Aichi virus 1 (AiV-1) is a human pathogen from the Kobuvirus genus of the Picornaviridae family. Unlike most picornaviruses, kobuvirus capsids are composed of only three types of subunits: VP0, VP1, and VP3. The polyprotein is cotranslationally and posttranslationally cleaved into leader protein (L-protein), viral capsid proteins VP0, VP3, and VP1, and nonstructural proteins that control the replication of AiV-1 in the infected cell. The capsid is built from major capsid proteins VP0, VP1, and VP3 arranged with pseudo-T3 icosahedral symmetry.

AiV-1 virions released their RNA rather abruptly at 53°C. Electron microscopy of AiV-1 virions heated to 53°C for 10 min identified 95% of empty capsids, which were used to reconstruct the empty particle to a resolution of 4.2 Å. The AiV-1 empty capsid is expanded by 7.6 Å in diameter relative to the native virus. The structure of the empty particle differs from that of the native virion, mostly in the contacts between the pentamers of capsid protein protomers. In the native AiV-1 virion, the interpentamer contacts are mediated by strand β2 of VP0, which interacts with β-strand F of VP3. However, in the empty particle residues 112 to 139, which form the β1 and β2 strands of VP0, are disordered. As a consequence, the interpentamer interface is reduced from 2,750 to 1,400 Å2. At the same time, residues 55 to 60 of VP0 became structured in the empty AiV-1 particle and residues 67 to 75 retain the same structure as in the native virions. Therefore, the N-terminal arm of AiV-1 VP0 does not appear to be externalized from the empty particle. The N-terminal arm of AiV-1 VP1 undergoes structural reorganization upon the formation of the empty particle. Residues 1 to 30 become disordered, and residues 31 to 35 refold into a new structure with the last resolved residue pointing toward the particle center.

> TLTEDLDAPQDTGNIENGAADNSPQPRTTFDYTGNPLPPDTKLENFFSFYRLLPMGGSGAPSLSFPADEGTIIPLNPINWLKGADVSGIAAMLSCFTYIAADLRITLRFSNPNDNPATMLVAFAPPGATIPLKPTRQMLSNFYMAEVPVSAATSTMVSFSIPYTSPLSAIPTSYFGWEDWSGTNFGQLSSGSWGNLMLIPSLSVDSAIPFDFQLSCWVAFGNFKAWVPRPPPPLPPLPTPAANAERTVAVIKQ;> GNSVTNIYGNGNNVTTDVGANGWAPTVSTGLGDGPVSASADSLPGRSGGASSEKTHTVSGSSNKVGSRFSKWWEPAAARASESATDSAIEGIDAAGKAASKAITRKLDRPAAPSSTANPQPSLIALNPSATQSGNASILTGSTAPSLLAYPTATPVPLPNPDEPSQPGPSGDRTWLLDTVTWSQEFTRGWNIAGSNGMQWTGLESLIFPVSTDTNWTSTSSPTAYPLPFSFVRAYPDSSWAAMYNTHSMWNCGWRVQVTVNGSQFHAGALILYMVPEATTHAIQTARDNAGFVFPYVILNLYESNTATIEVPYISPTPNTSSGLHAPWTFYLQVLSPLNPPPSLPTSLSCSIYVTPVDSSFHGLRYLAPQ;> HWKTRAVPGAGTFGSAVAGQELPLCGVRAYYPPNAYIPAQVRDWLEFAHRPGLMATVPWTMADEPAERLGIFPVSPSAIAGTGAPISYVISLFSQWRGELAAHLLFTGSAQHYGRLVVCYTPAAPQPPSTMQEAMRGTYTVWDVNAASTLEFTIPFISNSYWKTVDVNNPDALLSTTGYVSIWVQNPLVGPHTAPASALVQAFISAGESFNVRLMQNPALTSQ>[2x]MKQYLELMQKVLDEGTQKNDRTGTGTLSIFGHQMRFNLQDGFPLVTTKRCHLRSIIHELLWFLQGDTNIAYLHENNVTIWDE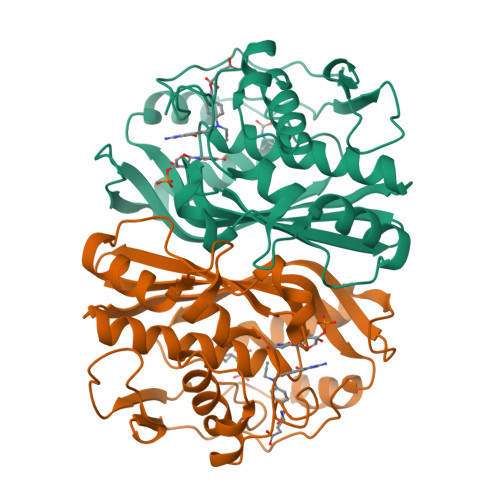WADENGDLGPVYGKQWRAWPTPDGRHIDQITTVLNQLKNDPDSRRIIVSAWNVGELDKMALAPCHAFFQFYVADGKLSCQLYQRSCDVFLGLPFNIASYALLVHMMAQQCDLEVGDFVWTGGDTHLYSNHMDQTHLQLSREPRPLPKLIIKRKPESIFDYRFEDFEIEGYDPHPGIKAPVA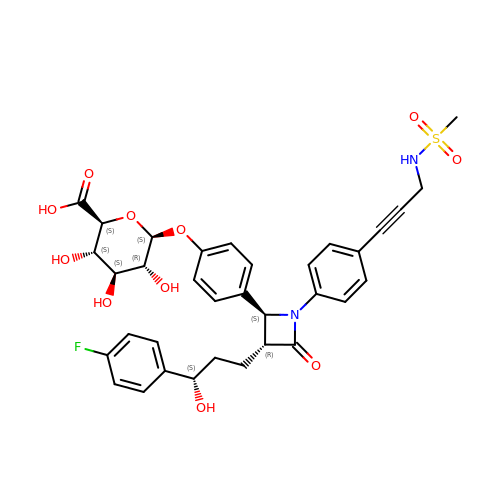4-[(2S,3R)-3-[(3S)-3-(4-fluorophenyl)-3-hydroxypropyl]-1-(4-{3-[(methylsulfonyl)amino]prop-1-yn-1-yl}phenyl)-4-oxoazetidin-2-yl]phenyl beta-D-glucopyranosiduronic acid | C34 H35 F N2 O11 S | DWURZHBEXYXPMW-WHTAKPIKSA-N PRPP is formed from ATP and D-ribose-5-phosphate (R5P) by the phosphoribosyl pyrophosphate synthetases (PRSs). The human PRS family, which has 3 isoforms (hPRS1, hPRS2 and hPRS3), belongs to the class I PRSs that requires divalent metal ions such as Mg2+ as the activator, inorganic phosphate ion for activity, and ATP or dATP as the diphosphoryl donor. Due to the important role of PRPP in the nucleotide metabolic process, the stability of PRPP content is essential for cell physiology and is predominantly controlled by hPRS1, the ubiquitously expressed human PRPP synthetase. Mutations in hPRS1 affect vital cell functions and are related to many diseases and disorders.

We determined the crystal structures of the E43T, D65N, A87T, M115T and Q133P mutations at a resolution of 3.0 Å, 2.14 Å, 3.3 Å, 2.11 Å and 2.74 Å, respectively, with 2 molecules in each asymmetric unit. Overall, the structures of all the five structures are highly similar to that of the wild type PRS1 with RMSD listed in S2 Table. In the A87T and M115T structures, the mutations of hydrophobic residues decrease the hydrophobic character of both Ala87 and Met115. In the PRS1 structure, Ala87 is located in the hydrophobic core of the N-terminal domain, whereas Met115 is located at the hydrophobic A-B dimer interface. Consequently, the M115T mutation might affect the A-B dimerization interface, whereas the A87T mutation might slightly affect the secondary structural elements of the N terminal domain. Approximately 31% of these mutations have hydrophobic side chains and low solvent accessibilities, such as A87T, L129I, V142L, L152P and I290T. These mutations might disrupt the secondary structure at given sites, and may interfere with the hydrophobic interaction of the secondary structure elements, which stabilize the protein quaternary structure.

>[2x]MPNIKIFSGSSHQDLSQKIADRLGLELGKVVTKKFSNQETCVEIGESVRGEDVYIVQSGCGEINDNLMELLIMINACKIASASRVTTVIPCFPYARQDKKDKSRAPISAKLVANMLSVAGADHIITMDLHASQIQGFFDIPVDNLYAEPAVLKWIRENISEWRNCTIVSPDAGGAKRVTSIADRLNVDFALIHKERKKANEVDRMVLVGDVKDRVAILVDDMADTCGTICHAADKLLSAGATRVYAILTHGIFSGPAISRINNACFEAVVVTNTIPQEDKMKHCSKIQVIDISMILAEAIRRTHNGESVSYLFSHVPLLEHHHHHH>MSLTSGEQAKTPL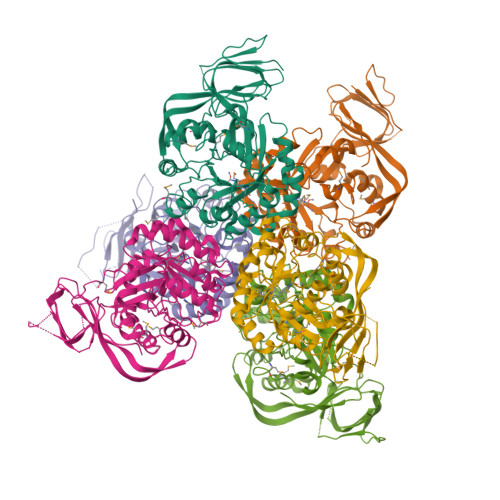QAPILLTNVKPVGFGKGASQSSTDILIGGDGKIAAVGSALQAPADTQRIDAKGAFISPGWVDLHVHIWHGGTDISIRPSECGAERGVTTLVDAGSAGEANFHGFREYIIEPSRERIKAFLNLGSIGLVACNRVPELRDIKDIDLDRILECYAENSEHIVGLKVRASHVITGSWGVTPVKLGKKIAKILKVPMMVHVGEPPALYDEVLEILGPGDVVTHCFNGKSGSSIMEDEDLFNLAERCAGEGIRLDIGHGGASFSFKVAEAAIARGLLPFSISTDLHGHSMNFPVWDLATTMSKLLSVDMPFENVVEAVTRNPASVIRLDMENRLDVGQRADFTVFDLVDADLEATDSNGDVSRLKRLFEPRYAVIGAEAIAASRYIPRARKLVRHSHGYSWREGHHHHHH[6x]>MVLYFIGLGLYDERDITVKGLEIAKKCDYVFAEFYTSLMAGTTLGRIQKLIGKEIRVLSREDVELNFENIVLPLAKENDVAFLTPGDPLVATTHAELRIRAKRAGVESYVIHAPSIYSAVGITGLMIYKFGKSATVAYPEGNWFPTSYYDVIKENAERGLHTLLFLDIKAEKRMYMTANEAMELLLKVEDMKKGGVFTDDTLVVVLA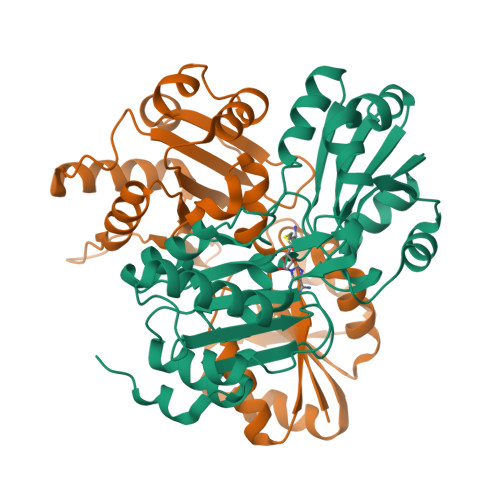RAGSLNPTIRAGYVKDLIREDFGDPPHILIVPGKLHIVEAEYLVEIAGAPREILRVNV[2x]>[4x]MNEEEKIKNDMLKYIEKDPKIGVWSYPAFLVL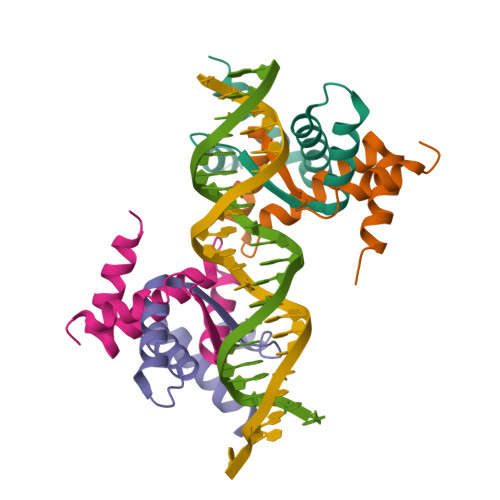QYLYHTVPGFKMSRTAKEALEKGLKEMYPTLFTIAEKIAKERFKEHHHHHH> TDTTNSIKHVISPLARQTLQDRDLTRPVAGKRPIRLLPWLQVVKIGGRVMDRGADAILPLVEELRKLLPEHRLLILTGAGVRARHVFSVGLDLGLPVGSLAPLAASEAGQNGHILAAMLASEGVSYVEHPTVADQLAIHLSATRAVVGSAFPPYAHHEFPGSRIPPHRADTGAFLLADA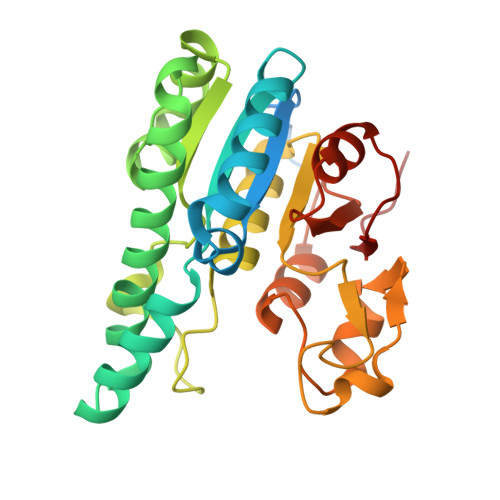FGAAGLTIVENVDGIYTADPNGPDRGQARFLPETSATDLAKSEGPLPVDRALLDVMATARHIERVQVVNGLVPGRLTAALRGEHVGTLIRTGVRPA> MRGSHHHHHHGMASMELSSLTAVSPVDGRYGDKVSALRGIFSEYGLLKFRVQVEVRWLQKLAAHAAIKEVPAFAADANGYLDTLVANFNEEDAARIKTIERTTNHDVKAVEYFLKEKVAAIPALHDVSEFIHFACTSE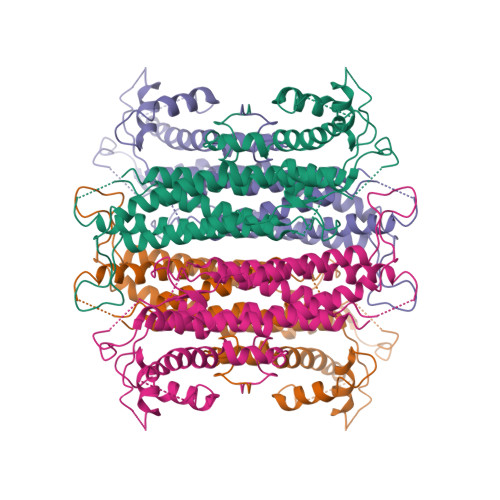DINNLSHALMLKTARDEVILPYWRQVINAVKDLATQYRDIPLLSRTHGQPATPSTLGKEMANVAYRMERQFRQLNQVEILGKINGAVGNYNAHIAAYPEVDWHQFSEEFVTSLGIQWNPYTTQIEPHDYIAELFDCIARFNTILIDFDRDVWGYIALNHFKQKTIAGEIGSSTMPHKVNPIDFENSEGNLGLSNAVLHHLANKLPVSRWQRDLTDSTVLRNLGVGIGYALIAYQSTLKGVSK> ICVNENGGCEQYCSDH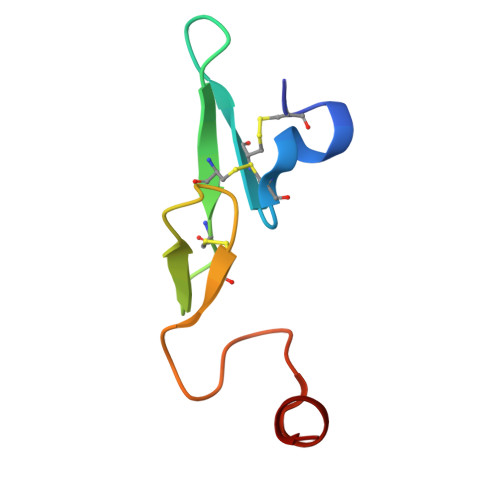TGTKRSCRCHEGYSLLADGVSCTPTVEYPCGKIPILEKR>[2x]SMSATLILEPPGRCCWNEPVRIAVRGLAPEQRVTLRASLRDEKGALFRAHARYCADACGELDLERAPALGGSFAGLEPMGLLWALEPEKPFWRFLKRDVQIPFVVELEVLDGHDPEPGRLLCQAQHERHFLPPGVWRQSVRAGRVRATLFLPPGPGPFPGIIDIFGIGGGLLEYRASLLAGHGFATLALAYYNFEDLPNNMDNISLEYFEEAVCYMLQHPQVKGPGIGLLGISLGADICLSMA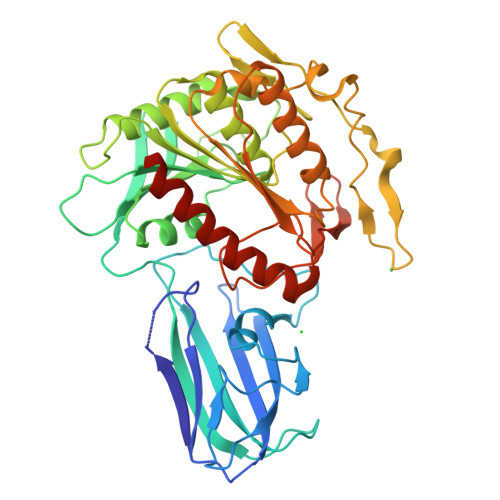SFLKNVSATVSINGSGISGNTAINYKHSSIPPLGYDLRRIKVAFSGLVDIVDIRNALVGGYKNPSMIPIEKAQGPILLIVGQDDHNWRSELYAQTVSERLQAHGKEKPQIICYPGTGHYIEPPYFPLCPASLHRLLNKHVIWGGEPRAHSKAQEDAWKQILAFFCKHLGGTQKTAVPKL> GAHMDCHLSDMLQQLHSVNASKPS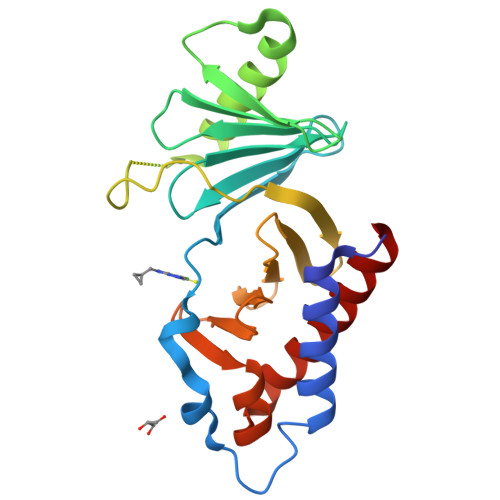ERGLVRQEEAEDPACIPIFWVSKWVDYSDKYGLGYQLCDNSVGVLFNDSTRLILYNDGDSLQYIERDGTESYLTVSSHPNSLMKKITLLKYFRNYMSEHLLKAGANITPREGDELARLPYLRTWFRTRSAIILHLSNGSVQINFFQDHTKLILCPLMAAVTYIDEKRDFRTYRLSLLEEYGCCKELASRLRYARTMVDKLLSSR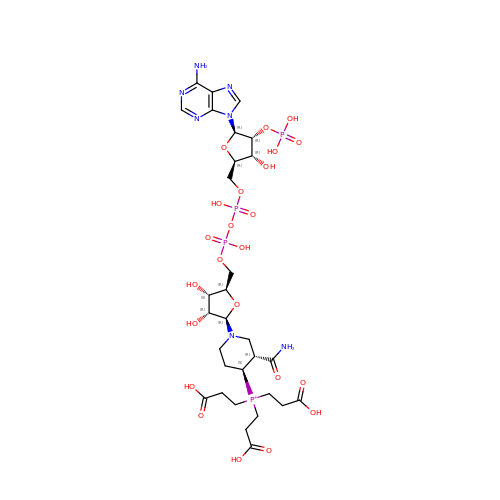[(4~{S})-3-aminocarbonyl-1-[(2~{R},3~{R},4~{S},5~{R})-5-[[[[(2~{R},3~{R},4~{R},5~{R})-5-(6-aminopurin-9-yl)-3-oxidanyl-4-phosphonooxy-oxolan-2-yl]methoxy-oxidanyl-phosphoryl]oxy-oxidanyl-phosphoryl]oxymethyl]-3,4-bis(oxidanyl)oxolan-2-yl]piperidin-4-yl]-tris(3-hydroxy-3-oxopropyl)phosphanium | C30 H48 N7 O23 P4 | KCEMQRAWVXDPSM-NLJDEQFRSA-O> APDTSSSNKQNFSTDVIYQIFTDRFSDGNPANNPTGAAFDGTCTNLRLYCGGDWQGIINKINDGYLTGMGVTAIWISQPVENIYSIINYSGVNNTAYHGYWARDFKKTNPAYGTIADFQNLIAAAHAKNIKVIIDFAPNHTSPASSDQPSFAE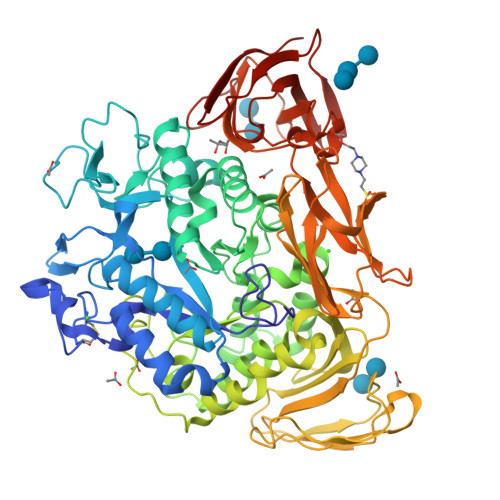NGRLYDNGTLLGGYTNDTQNLFHHNGGTDFSTTENGIYKNLYDLADLNHNNSTVDVYLKDAIKMWLDLGIDGIRMDVVKHMPFGWQKSFMAAVNNYKPVFTFGEWFLGVNEVSPENHKFANESGMSLLDFRFAQKVRQVFRDNTDNMYGLKAMLEGSAADYAQVDDQVTFIDNHDMERFHASNANRRKLEQALAFTLTSRGVPAIYYGTEQYMSGGTDPDNRARIPSFSTSTTAYQVIQKLAPLRKSNPAIAYGSTQERWINNDVLIYERKFGSNVAVVAVNRNLNAPASISGLVTSLPQGSYNDVLGGLLNGNTLSVGSGGAASNFTLAAGGTAVWQYTAATATPTIGHVGPMMAKPGVTITIDGRGFGSSKGTVYFGTTAVSGADITSWEDTQIKVKIPAVAGGNYNIKVANAAGTASNVYDNFEVLSGDQVSVRFVVNNATTALGQNVYLTGSVSELGNWDPAKAIGPMYNQVVYQYPNWYYDVSVPAGKTIEFKFLKKQGSTATWEGGSNHTFTAPSSGTGTINVNWQP>SERFPNDVDPIETRDWLQAIESVIREEGVERAQYLIDQLLAEARKGGVNVAAGTGISNYINTIPVEEQPEYPGNLELERRIRSAIRWNAIMTVLRASKKDLELGGHMASFQSSATIYDVCFNHFFRARNEQDGGDLVYFQGHISPGVYARAFLEGRLTQEQLDNFRQEVHGNGLSSYPHPKLMPEFWQFPTVSMGLGPIGAIYQAKFLKYLEHRGLKDTSKQTVYAFLGDGEMDAPESKGAITIATREKLDNLVFVINCNLQRLDGPVTGNGKIINELEGIFEGAGWNVIKVMWGSRWDELLRKDTSGKLIQLMNETVDGDYQTFKSKDGAYVREHFFGKYPETAALVADWTDEQIWALNRGGHDPKKIYAAFKKAQETKGKATVILAHTIKGYGMGDAAEGKNIAHQVKKMNMDGVRHIRDRFNVPVSDADIEKLPYITFPEGSEEHTYLHAQRQKLHGYLPSRQPNFTEKLELPSLQDFGALLEEQSKEISTTIAFVRALNVMLKNKSIKDRLVPIIADEARTFGMEGLFRQIGIYSPNGQQYTPQDREQVAYYKEDEKGQILQEGIN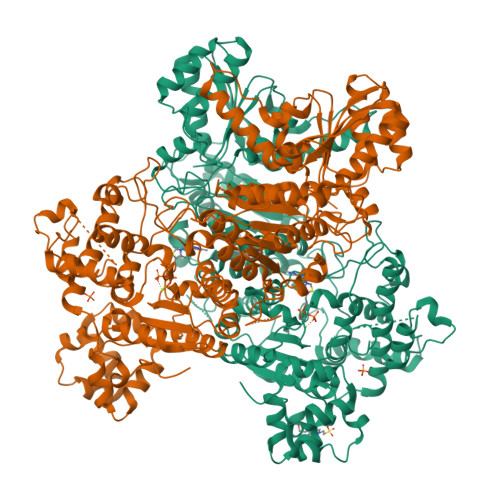ELGAGCSWLAAATSYSTNNLPMIPFYIYYSMFGFQRIGDLCWAAGDQQARGFLIGGTSGRTTLNGEGLQHEDGHSHIQSLTIPNCISYDPAYAYEVAVIMHDGLERMYGEKQENVYYYITTLNENYHMPAMPEGAEEGIRKGIYKLETIEGSKGKVQLLGSGSILRHVREAAEILAKDYGVGSDVYSVTSFTELARDGQDCERWNMLHPLETPRVPYIAQVMNDAPAVASTDYMKLFAEQVRTYVPADDYRVLGTDGFGRSDSRENLRHHFEVDASYVVVAALGELAKRGEIDKKVVADAIAKFNIDADKVNPRLA[2x]3,6-bis(3-(3'-(R)-fluoropyrrolindino)propionamido)acridine | C27 H31 F2 N5 O2 | 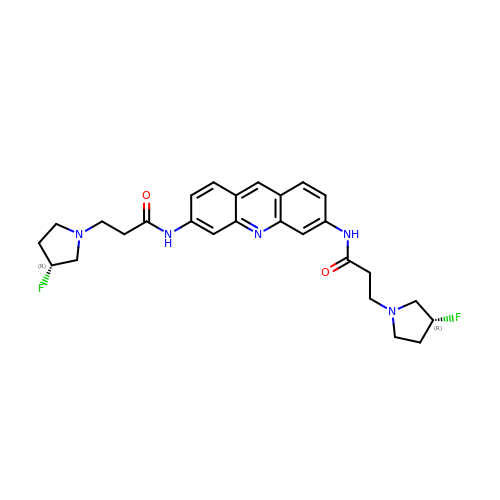LWWRDCOEZPEHNJ-NHCUHLMSSA-N> YEYYNELAENKTYKKLAIEAPRGEIKDRYGRLLAGNKNLFTVQVSGNDINKKDANKHSRANEISLKLINLLERNGEEYVDEFPIYVENGKYYYTYDRDIREYKSENGIPNDYNAKESFYYLVDKLISAGILSQEDKRLDATRLQAKLNENGYYPPILVSKWMFTAERDKRDWLASYKIKETKLSAKEAFEKVRNSDALEIDKSLSDEDARKIMVVRDLIKSKGYSQYNPVTIAKDVGETTIAQIEESAMDLVGVSIAVEPVRYYPNGSLASHMLGYVGKMPSTQIESYLQKGYETGDMVGLAGVEKSNESRLRGTDGYKMVKVDALGRISKEIESKKPKSGDTVYLTLDKDLQEVSDNALKQIIEVASKGGTFKSKFGDKPISAYAGKAQSAALIAIDVKNGEVLASSSYPNYDPNKFAKGISTEDYKALQPKNPNDLLAGSPLLNLVTQGEFQPGSSFKMLTSMAALENGLDPNFTINDPGVIMLGKKSFGDYVWNHGRGNHGMTNLYKAIQESCNIYMATIGTGKTWPDGKSIGIDMNANKILEYAKLFGLDQNTGLQDEVEERAGKVPSTEDKLKSTQALLKSNLEREMANDFVDITREKNPKEYEKRINEIVSWAAEKKTPGRVETMNRLKKMNVKEDRIEEVADLAVFSYFNFAKWSTADTFNLAIGQGENAYTPAQISRYVAAIANGGNLVELSVVDRAVSSDYSSVKINDQKKVEKIPFKNPDNLKELTKGMKLVARQGTAKSAFADFPIDVAAKTGTAEKSGKIPTDNEYEYLKSHMSSYNVNLNDAIKLADKMKAEKEKELSLAKEKEIKKKLENKDLKDEERKKLEEELEDGVKVRLEDTDKVNSSYLRKAIKELNPKITDDQIDRFKQDYGSFTWTVAFAPADDPEIAVVCVIPQGDSSVFSLLPTREVIGTYMGL

Cephalosporins are members of the β-lactam family of antibiotics. These drugs achieve their bactericidal potency by irreversibly inhibiting penicillin-binding proteins (PBPs), particularly the transpeptidase (TPase) PBPs that cross-link cell wall peptidoglycan. Four annotated TPase PBPs exist in the genome of C. difficile R20291, a hypervirulent epidemic ribotype 027 strain: PBP1 (CDR20291_0712), PBP2 (CDR20291_0985), PBP3 (CDR20291_1067), and SpoVD (CDR20291_2544). A recent study found PBP1 and PBP2 are essential for vegetative growth in R20291, while SpoVD and PBP3 are essential for sporogenesis. Remarkably, in addition to C. difficile PBP2, we find this Zn2+-binding motif is also present in C. difficile PBP3 and SpoVD, meaning three of the four TPase PBPs, and all three class B PBPs in C. difficile have this motif.

For the first time, we present its crystal structure with ampicillin at 3.0 Å resolution. The TPase domain adopts a canonical penicilloyl serine transferase fold, characterized by a five-stranded β-sheet that is sandwiched by three α-helices. The active site is found between the third, KTG-motif bearing strand of the five-stranded β-sheet (PBP numbering: β3 / overall: β15), an SXN motif across the channel, (S550-C551-N552) and two, nearly orthogonal α-helices that form the floor of the narrow substrate-binding cleft. One of these α-helices (α13) covalently binds to ampicillin through its catalytic S492. The crystal structure of PBP2 in complex with ampicillin at 3.0 Å resolution reveals three novel structural features. This includes a novel Zn2+-binding motif in the active site (bottom left), a charged, elongated, helix connecting the β3-β4 strands of the TPase domain, termed the “coiled-coil stretch” (bottom right), and five roughly parallel α-helices, the “central helical cluster”. The Zn2+ ion is coordinated by D515, D528, H538, and C551, where C551 is the X residue of the highly conserved SXN motif. However, the active site opens upon ampicillin binding, causing substrate-recognition residues to translate 1–2 Å outwards and the KTG-bearing β3 sheet to shift downward, rigidify, and displace the water molecule. These movements expose the catalytic serine, freeing it for nucleophilic attack. Interestingly, the putative MreC binding cleft formed at the NTD “hinge” splays at different angles between the ampicillin and unbound structures, exposing a hydrophobic crevasse that is significantly narrower when bound to ampicillin.The Staphylococcus aureus inosine triphosphate pyrophos­phatase is a dimeric enzyme that hydrolyses noncanonical nucleoside triphosphates to prevent their incorporation into DNA and RNA. Proteins are biological entities that present various degrees of flexibility reflecting their molecular functions. They can adopt different conformations to perform catalysis, ligand binding and allostery.

We obtained a crystal form of this enzyme in which the asymmetric unit contained a dimer consisting of one monomer in an open state and the other in a closed conformation upon binding of a phosphate molecule at the active site of the protein. For instance, the E. coli liganded dimer structure could not be solved by molecular replacement using the apo RdgB structure and was solved using the SAD method. Because we usually assume that there is only one overall conformation in a crystal, it could have been useful to compute the self-rotation in order to evaluate to what extent the conformations of the two monomers were different, with the highest divergence producing pseudo-symmetry peaks with lower correlation. For this peculiar case, using data between 15 and 4 Å resolution, the self-rotation produced a pseudo-symmetry peak with a 37.5% correlation. The height of the correlations of the self-rotation peaks corresponding to the NCS provides a hint to the conformational variability of the monomers (the correlation values being inversely proportional to the amplitude of the conformational differences). The same case can arise for oligomeric structures following the sequential model of allosteric regulation, in which different monomers can adopt different conformations in the same crystal.

>[2x]MKEIVIASNNQGKINDFKVIFPDYHVIGISELIPDFDVEETGSTFEENAILKSEAAAKALNKTVIADDSGLEVFALNGEPGIYSARYAGENKSDEANIEKLLNKLGNTTDRRAQFVCVISMSGPDMETKVFKGTVSGEIADGKYGENGFGYDPIFYVPKLDKTMAQLSKEQKGQISHRRNAINLLQAFLEGEKNV> MGEKLELRLKSPVGAEPAVYPWPLPVYDKHHDAAHE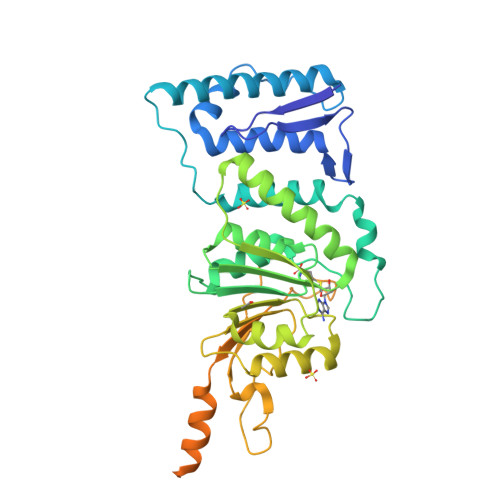IIETIRWVCEEIPDLKLAMENYVLIDYDTKSFESMQRLCDKYNRAIDSIHQLWKGTTQPMKLNTRPSTGLLRHILQQVYNHSVTDPEKLNNYEPFSPEVYGETSFDLVAQMIDEIKMTDDDLFVDLGSGVGQVVLQVAAATNCKHHYGVEKADIPAKYAETMDREFRKWMKWYGKKHAEYTLERGDFLSEEWRERIANTSVIFVNNFAFGPEVDHQLKERFANMKEGGRIVSSKPFAPLNFRINSRNLSDIGTIMRVVELSPLKGSVSWTGKPVSYYLHTIDRTILENYFSSLKNPKLREEQEAARRRQQRESKSNAATPTKGPEGKVAGPADAPMDSGAEEEKAGAATVKKPSPSKARKKKLNKKGRKMAGRKRGRPKK> GGA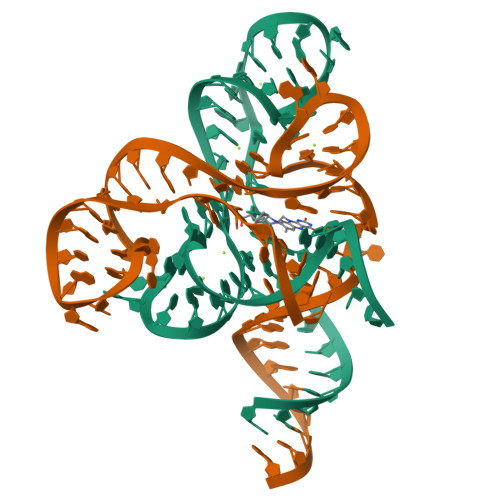UCUUCGGGGCAGGGUGAAAUUCCCGACCGGUGGUAUAGUCCACGAAUCCAU;> GGAUUGAUUUGGUGAAAUUCCAAAACCGACAGUAGAGUCUGGAUGAGAGAAGAUUCG>[2x]MKRVVITGLGIVSSIGNNQQEVLASLREGRSGITFSQELKDSGMRSHVWGNVKLDTTGLIDRKVVRFMSDASIYAFLSMEQAIADAGLSPEAYQNNPRVGLIAGSGGGSPRFQVFGADAMRGPRGLKAVGPYVVTKAMASGVSACLATPFKIHGVNYSISSASATSAHCIGNAVEQIQLGKQDIVFAGGGEELCWEMACEFDAMGALSTKYNDTPEKASRTYDAHRDGFVIAGGGGMVVVEELEHALARGAHIYAEIVGYGATSDGADMVAPSGEGAVRCMKMAMHGVDTPIDYLNSHGTSTPVGDVKELAAIREVFGDKSPAISATKAMTGHSLGAAGVQEAIYSLLMLEHGFIAPSINIEELDEQAAGLNIVTETTDRELTTVMSNSFGFGGTNATLVMRKLKD;>MLVLVAPGQGAQTPGFLTDWLALPGAADRVAAWSDAIGLDLAHFGTKADADEIRDTSVAQPLLVAAGILSAAALGTGFTPGAVAGHSVGEITAAVFAGVLDDTAALSLVRRRGLAMAEAAAVTETGMSALLGGDPEVSVAHLERLGLTPANVNGAGQIVAAGTMEQLAALNEDKPEGVRKVVPLKVAGAFHTRHMAPAVDKLAEAAKALTPADPKVTYVSNKDGRAVASGTEVLDRLVGQVANPVRWDLCMETFKELGVTAIIEVCPGGTLTGLAKRALPGVKTLALKTPDDLDAARELVAEHT[2x];>[2x]VDKRESYTKEDLLASGRGELFGAKGPQLPAPNMLMMDRVVKMTETGG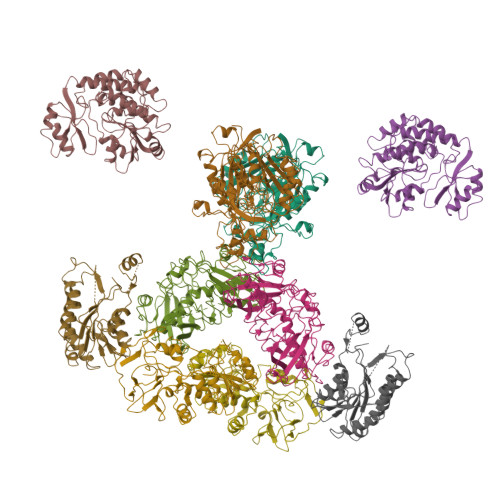NFDKGYVEAELDINPDLWFFGCHFIGDPVMPGCLGLDAMWQLVGFYLGWLGGEGKGRALGVGEVKFTGQVLPTAKKVTYRIHFKRIVNRRLIMGLADGEVLVDGRLIYTASDLKVGLFQDTSAFVDKRESYTKEDLLASGRGELFGAKGPQLPAPNMLMMDRVVKMTETGGNFDKGYVEAELDINPDLWFFGCHFIGDPVMPGCLGLDAMWQLVGFYLGWLGGEGKGRALGVGEVKFTGQVLPTAKKVTYRIHFKRIVNRRLIMGLADGEVLVDGRLIYTASDLKVGLFQDTSAF;>MKAWVLKRLGGPLELVDLPEPEAEEGEVVLRVEAVGLNFADHLMRLGAYLTRLHPPFIPGMEVVGVVEGRRYAALVPQGGLAERVAVPKGALLPLPEGLSPEEAAAFPVSFLTAYLALKRAQARPGEKVLVQAAAGALGTAAVQVARAMGLRVLAAASRPEKLALPLALGAEEAATYAEVPERAKAWGGLDLVLEVRGKEVEESLGLLAHGGRLVYIAPIPPLRLMRRNLAVLGFWLTPLLREGALVEEALGFLLPRLGRELRPVVGPVFPFAEAEAAFRALLDRGHTGKVVVRL[2x];>[2x]MNFEGKIALVTGASRGIGRAIAETLAARGAKVIGTATSENGAQAISDYLGANGKGLMLNVTDPASIESVLEKIRAEFGEVDILVNNAGITRDNLLMRMKDEEWNDIIETNLSSVFRLSKAVMRAMMKKRHGRIITIGGQANYAAAKAGLIGFSKSLAREVASRGITVNVVAPGFIETSDDQRAGILAQVPAGRLGGAQEIANAVAFLASDEAAYITGETLHVNGGM> MAVKVEYDLKRLRNIGIAAHIDAGKTTTTERILYYTGRIHKIGEVHEGAATMDFMEQERERGITITAAVTTCFWKDHRINIIDAPGHVDFTIEVERSMRVLDGAIVVFDSSQGVEPQSETVWRQAEKYKVPRIAFANKMDKTGADLWLVIRTMQERLGARPVVMQLPIGREDTFSGIIDVLRMKAYTYGNDLGTDIREIPIPEEYLDQAREYHEK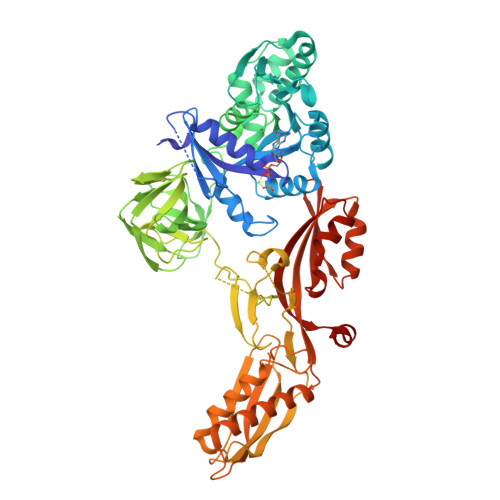LVEVAADFDENIMLKYLEGEEPTEEELVAAIRKGTIDLKITPVFLGSALKNKGVQLLLDAVVDYLPSPLDIPPIKGTTPEGEVVEIHPDPNGPLAALAFKIMADPYVGRLTFIRVYSGTLTSGSYVYNTTKGRKERVARLLRMHANHREEVEELKAGDLGAVVGLKETITGDTLVGEDAPRVILESIEVPEPVIDVAIEPKTKADQEKLSQALARLAEESPTFSVSTHPETGSTIISGMGELSLEIIVDRLKREFKVDANVGKPQVAYRETITKPVDVEGKFIRQTGGRGQYGHVKIKVEPLPRGSGFEFVNAIVGGVIPKEYIPAVQKGIEEAMQSGPLIGFPVVDIKVTLYDGSYHEVDSSEMAFKIAGSMAIKEAVQKGDPVILEPIMRVEVTTPEEYMGDVIGDLNARRGQILGMEPRGNAQVIRAFVPLAEMFGYATDLRSKTQGRGSFVMFFDHYQEVPKQVQEKLIKGQ RET receptor tyrosine kinase plays vital developmental and neuroprotective roles in metazoans. GDNF family ligands (GFLs) when bound to cognate GFRα co-receptors recognize and activate RET stimulating its cytoplasmic kinase function. The bipartite GFL-GFR complexes are recognized by the RET receptor tyrosine kinase (RTK) forming ternary RET-GFL-GFR complexes (Cacalano et al., 1998; Durbec et al., 1996; Jing et al., 1996; Treanor et al., 1996). RET has four consecutive cadherin-like domains (CLD(1-4)) and a membrane-proximal cysteine-rich domain (CRD) in its extracellular domain (RETECD) (Anders et al., 2001).

A reconstituted complex was assembled consisting of the zRETECD (residues 1–627), a C-terminal truncated zGFRα1a (zGFRα1aD1-3) covering residues 1–353, and an N-terminal truncated zGDNF, residues 135–235 (zGDNFmat.), defined hereafter as zRGα1a from RET-GDNF-GFRα1a. An initial cryo-EM dataset collected on the reconstituted zRGα1a yielded a 3D cryo-EM map that confirmed a 2:2:2 stoichiometry, consistent with size-exclusion multi-angle laser light scattering data and similar to recently published human RET complexes (Bigalke et al., 2019; Li et al., 2019). Additional processing with symmetry expansion in RELION-3 (Kimanius et al., 2016; Scheres, 2012; Zivanov et al., 2018), improved the anisotropy and resolution of the map by addressing flexibility at the 2-fold symmetry axis, to produce a map with a nominal resolution of 3.5 Å. The final structure shows zGDNF at the core of the complex flanked by two zGFRα1aD1-3 co-receptors, both of which are further enveloped by two “G”-shaped RETECD molecules. There are two major interfaces between zRETECD and its ligand-co-receptor at opposite ends of zRETECD, each is well defined in the cryo-EM map with side-chain level information. The dominant interaction is between zCLD(1-3) and GFRα1D3 (defined hereafter as the site 1), with a key second site between zCRD and a concave surface presented by the GDNF dimer and a loop from GFRα1 (defined hereafter as site 2). Comparison of site 1 of zRET in both the crystal and cryo-EM structure reveals differences in the conformation of residues 288–298 from a CLD3 loop. In the presence of the ligand, this loop forms a central part of the interface with zGFRα1aD3 and is repositioned upward (loop-“up”) toward the calcium ions and engages L247 of helix α1 of zGFRα1aD2. Comparison of all available liganded RETECD structures at site 2 consistently show a spacing of 44.2–47.0 Å between each pair of CRD C termini (measured at residue E613/620 in zRET/hRET) within an RET dimer. Upon closer inspection using RELION particle reposition (Zivanov et al., 2018) a homotypic interaction between zRGα1a particles was observed throughout the grids resulting in linear arrays of complexes.

>GLYFPQRLYTENIYVGQQQGSPLLQVISMREFPTERPYFFLCSHRDAFTSWFHIDEASGVLYLNKTLEWSDFSSLRSGSVRSPKDLTLKVGVSSTPPMKVMCTILPTVEVKLSFINDTAPSCGQVELSTLCFPEKISNPHITENREPGALRQLRRFTHMSICPNYTISYGVVAGSSVPFAVDDSTSELVVTAQVDREEKEVYHLDIVCMVRTERNLEEVFRSLHVNIYDEDDNSPYVNGTDTEDVLVEFDRSEGTVFGTLFVYDRDTTPVYPTNQVQNKLVGTLMTNDSWIKNNFAIEHKFREEKAIFGNVRGTVHEYKLKLSQNLSVTEQRSFLLGYLVNDTTFPGPEGTVLLHFNVTVLPVPIRFSNVTYSFTVSQKATTYSQIGKVCVENCQKFKGIDVTYQLEIVDRNITAEAQSCYWAVSLAQNPNDNTGVLYVNDTKVLRRPECQELEYVVIAQEQQNKLQAKTQLTVSFQGEADSLRTDEPRFPACAEKRQRGDCEATRGLGAPTGRCQWRQGRDKGISKRYSTCSPNLGTCPDGYCDAIESKNISICPQDCSSEAIIGGYERDLYGIKAGHGTCYCFEGKCFCERDEPEDDICNDMCGSEFENLYFQ[2x];>[2x]EESYFSSSNRLDCVKANELCLKEPGCSSKYRTMRQCVAGRESNFSMATGMEAKDECRLVLDALKQSPLYNCRCKRGMKKEKNCLRIYWGIYQHLQGNDLLEDSPYEPVNSRLSDIFRLAPIYSGEPALAKENNCLNAAKACNLNDTCKKYRSAYISPCTSRVSTAEVCNKRKCHKALRQFFDKVPPKHSYGMLYCSCPLGDQSACSERRRQTIVPACSYEDKERPNCLTLQVSCKTNYICRSRLADFFTNCQPEPLSLSGCLKENYADCLLSYSGLIGTVMTPNYLRSPKISVSPFCDCSSSGNSKEECDRFTEFFTDNACLRNAIQAFGNGGSEFLEVLFQGPGGGENLYFQ;>VKGQGRGCLLKEIHLNVTDLDLGYRTKEELIFRYCSGPCHDAETNYDKILNNLTHNKKLDKDTPSRTCCRPIAFDDDISFLDDSLEYHTLKKHSAKKCACV[2x]>[2x]GAPAEDQDCGRLPDFIAKLTNNTHQHVFDDLSGSVSLSWVGDSTGVILVLTTFQVPLVIVSFGQSKLYRSEDYGKNFKDITNLINNTFIRTEFGMAIGPENSGKVILTAEVSGGSRGGRVFRSSDFAKNFVQTDLPFHPLTQMMYSPQNSDYLLALSTENGLWVSKNFGEKWEEIHKAVCLAKWGPNNIIFFTTHVNGSCKADLGALELWRTSDL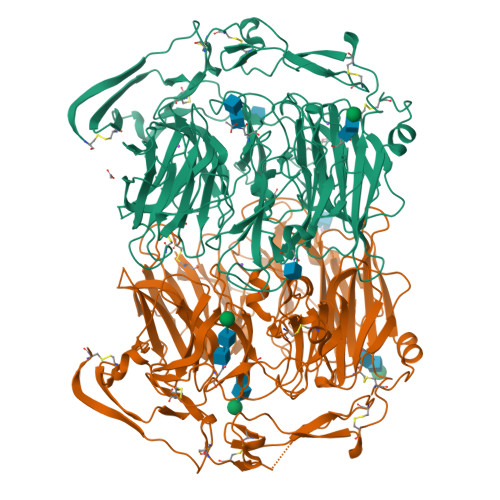GKTFKTIGVKIYSFGLGGRFLFASVMADKDTTRRIHVSTDQGDTWSMAQLPSVGQEQFYSILAANEDMVFMHVDEPGDTGFGTIFTSDDRGIVYSKSLDRHLYTTTGGETDFTNVTSLRGVYITSTLSEDNSIQSMITFDQGGRWEHLRKPENSKCDATAKNKNECSLHIHASYSISQKLNVPMAPLSEPNAVGIVIAHGSVGDAISVMVPDVYISDDGGYSWAKMLEGPHYYTILDSGGIIVAIEHSNRPINVIKFSTDEGQCWQSYVFTQEPIYFTGLASEPGARSMNISIWGFTESFITRQWVSYTVDFKDILERNCEEDDYTTWLAHSTDPGDYKDGCILGYKEQFLRLRKSSVCQNGRDYVVAKQPSVCPCSLEDFLCDFGYFRPENASECVEQPELKGHELEFCLYGKEEHLTTNGYRKIPGDKCQGGMNPAREVKDLKKKCTSNFLNIEGRHHHHHH>MSVKTWR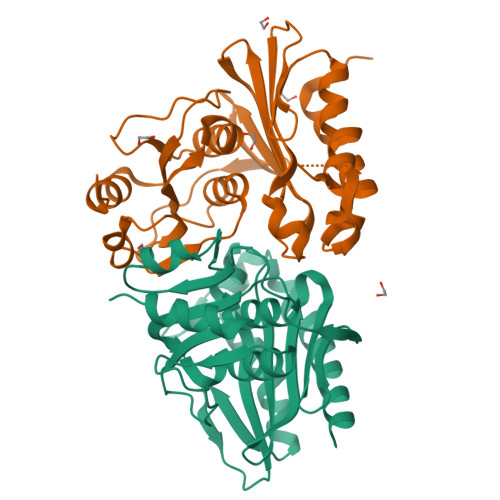KIAIDIIRDFDHNIMPLFGNPKASETISISPSGDETKVVDKVAENIIISKFKDLGVNVVSEEIGRIDQGSDYTVVVDPLDGSYNFINGIPFFAVSVAIFHEKDPIYAFIYEPIVERLYEGIPGKGSYLNGEKIKVRELAEKPSISFYTKGKGTKIIDKVKRTRTLGAIALELAYLARGALDAVVDIRNYLRPTDIAAGVVIAREAGAIVKDLDGKDVEITFSATEKVNIIAANNEELLETILRSIEK[2x]>[3x]KLKEIENRTRKPFEELCTELADLDMPAENIVLNRRVGQGAFGLVFGGEAKKSDLWEAVAVKVINEKANYEGKIDFLSEAKLMRSLNHPNVVRLIGISLNPKASLYLIMELMLLGDLKTYLLSRRILAQRSPNHEDIRPSTLTQMSMDIGQGLAYLHSKHLIHRDIACRNCLVAADRTVKIGDFGLTRQAAK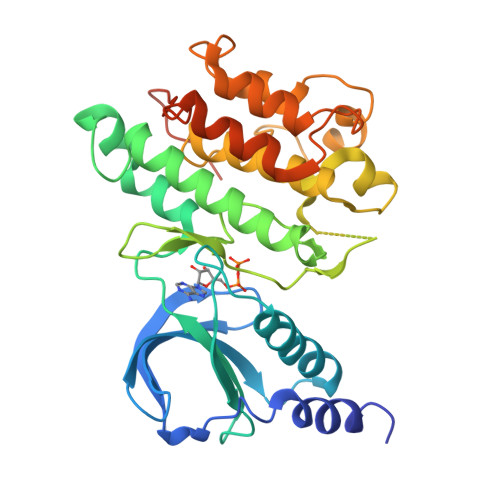NTSEAYYRFTRKCELPIRWMSPEAVQFGVFSIQSDIWSFGITLYEIITFGVFPYNGLGDVEVVERVKRMEFSITEFLPPQALNTVVCELINHCCKHQWQHRPSSMNQVLEVLIAYPDCIRPFLTDDPPKPNTTIDSLPFQPTVDTCIISE>MEAAASEPSLDLDNLKLLELIGRGRYGAVYKGSLDERPVAVKVFSFANRQNFINEKNIYRVPLMEHDNIARFIVGDERVTADGRMEYLLVMEYYPNGSLCKYLSLHTSDWVSSCRLAHSVTRGLAYLHTELPRGDHYKPAISHRDLNSRNVLVKNDGTCVISDFGLSMRLTGNRLVRPGEEDNAAISEVGTIRYMAPEVLEGAVNLRDCESALKQVDMYALGLIYWEIFMRCTDLFPGESVPEYQMAFQTEVGNHP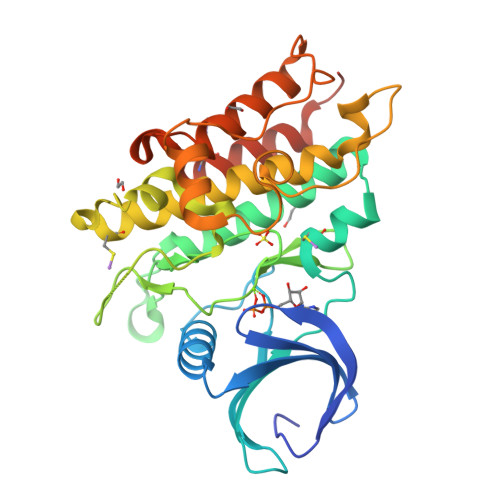TFEDMQVLVSREKQRPKFPEAWKENSLAVRSLKETIEDCWDQDAEARLTAQCAEERMAELMMIWERNKSVSPTAHHHHHH[2x]>EVVLLDFAAAGGELGWLTHPYGKGWDLMQNIMNDMPIYMYSVCNVMSGDQDNWL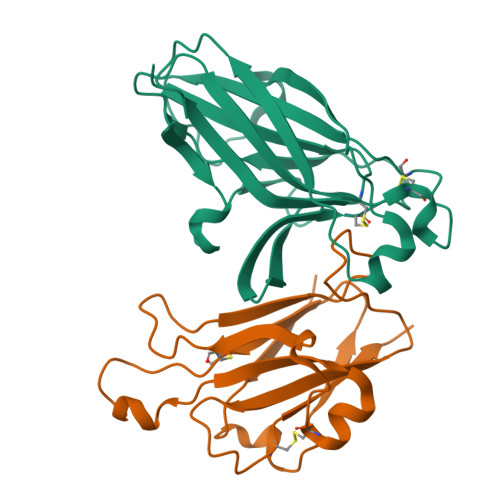RTNWVYRGEAERIFIELKFTVRDCNSFPGGASSCKETFNLYYAESDLDYGTNFQKRLFTKIDTIAPDEITVSSDFEARHVKLNVEERSVGPLTRKGFYLAFQDIGACVALLSVRVYYKKC[8x];>ADRHTVFWNSSNPKFRNEDYTIHVQLNDYVDIICPHYEDHSVADAAMEQYILYLVEHEEYQLCQPQSKDQVRWQCNRPSAKHGPEKLSEKFQRFTPFTLGKEFKEGHSYYYISKPIHQHEDRCLRLKVTVKI[8x]Family VIII esterases present similarities to class C β‐lactamases, which show nucleophilic serines located at the S‐X‐X‐K motif instead of the G‐X‐S‐X‐G or G‐D‐S‐(L) motif shown by other carboxylesterase families. Indeed, the analysis of the substrate specificity revealed its capacity to hydrolyse nitrocefin as a model chromogenic cephalosporin substrate (40.4 ± 11.4 units·g−1), and a large battery of 66 structurally different esters (up to 1730 min−1), including bis(2‐hydroxyethyl)‐terephthalate (241.7 ± 8.5 units·g−1) and the mycotoxin T‐2 (1220 ± 52 units·g−1). It also showed acyltransferase activity through the synthesis of benzyl 3‐oxobutanoate (40.4 ± 11.4 units·g−1) from benzyl alcohol and vinyl acetoacetate.

Structural analyses of free and substrate‐bound forms of this homooctamer esterase suggest that EH7 presents a more opened and exposed S1 site having no steric hindrance for the entrance of substrates to the active site, more flexible R1, R2 and R3 regions allowing for the binding of a wide spectrum of substrates into the active site, and small residues in the conserved motif Y‐X‐X containing the catalytic Tyr enabling the entrance of large substrates. These unique structural elements in combination with docking experiments allowed us to gain valuable insights into the substrate specificity of this esterase and possible others belonging to family VIII.

>MHHHHHHHHHHLEVLFQGPSEFPMAQSNIIAGMDLNRLDRIAEHLDRAYLHPGKLAGTMTLVARRGEVVYCQAQGLRDVERQLPVERDTLFRIYSMTKPITSIALMQLYEQGRFLLDEPVHKYIPTWKNLRVYKTGSHPQMLTTAPQRPMTIRDLLTHQSGLTYGFMNRTNVDAAYRSLKLDGGPGHTLDRLIDELARLPLEFSPGTAWNYSVATDVCGYLVQLLSGMSLDDYFSKHIFQPLGMPDTFFTVPAEKLSRFAACYEYQPGDSFSLQDDPQGSAFAKAHGYLSGGGGLVSCVDDYYRFAQALANGGELDGARIIGRKTLEFMRMNHLPDNKGLPDVAIGSFSETPYDGTGFGLGFSVKLDVAKSQTVGSVGEYGWGGMASTNFFIDPEEDLLMVFMTQLIPSSTYAVRQELRAIINGALVDA[8x]>DIFNRDPRDHYDLLQRLGGGTYGEVFKARDKVSGDLVALKMVKMEPDDDVSTLQKEILILKTCRHANIVAYHGSYLWLQKLWICMEFCGAGSLQDIYQVTGSLSELQISYVCREVLQGLAYLHSQKKIHRDIKGANILINDAGEVRLADFGISAQIGATLARRLSFIGTPYWMAPEVAAVALKGGYNE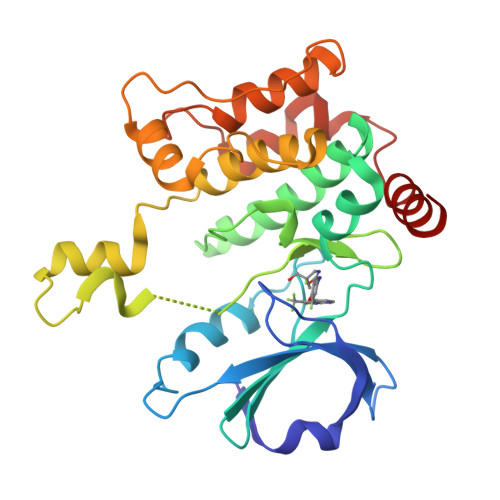LCDIWSLGITAIELAELQPPLFDVHPLRVLFLMTKSGYQPPRLKEKGKWSAAFHNFIKVTLTKSPKKRPSATKMLSHQLVSQPGLNRGLILDLLDKLKNP[2x]>ARSLLPLSTSLDHRSKEELHQDCLVLATAKHSRELNEDVSADVEERFHLGLF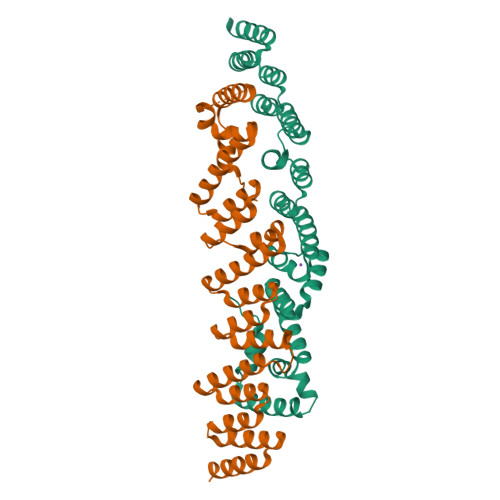TDRATLYRMIDIEGKGHLENGHPELFHQLMLWKGDLKGVLQTAAERGELTDNLVAMAPAAGYHVWLWAVEAFAKQLCFQDQYVKAASHLLSIHKVYEAVELLKSNHFYREAIAIAKARLRPEDPVLKDLYLSWGTVLERDGHYAVAAKCYLGATCAYDAAKVLAKKGDAASLRTAAELAAIVGEDELSASLALRCAQELL[2x]>SGQDLVPAAVEQAVPIQPVAGAALAAPAAGQINQIDPWIFQNFVQCPLGEFSISPRNTPGEILFDLALGPGLNPYLAHLSAMYTGWVGNMEVQLVLAGNAFTAGKVVVALVPPYFPKGSLTTAQITCFPHVMCDVRTLEPIQLPLLDVRRVLWHATQDQEESMRLVCMLYTPLRTNSPGDESFVVSGRLLSKPAADFNFVYLTPPIERTIYRMVDLPVIQPRLCTHARWPAPVYGLLVDPSLPSNPQWQNGRVHVDGTLLGTTPISGSWVSCFAAEAAYEFQSGTGEVATFTLIEQDGSAYVPGDRAAPLGYPDFSGQLEIEVQTETTKTGDKLKVTTFEMILG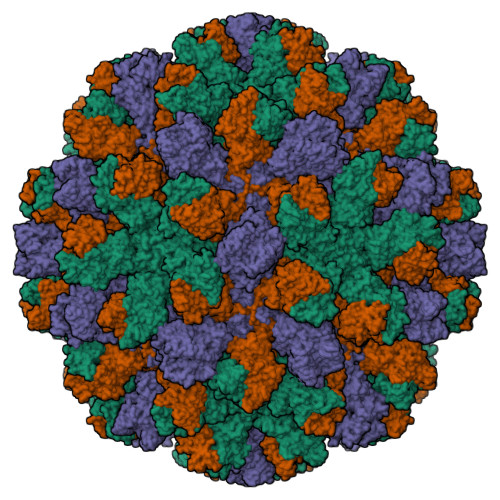PTTNADQAPYQGRVFASVTAAASLDLVDGRVRAVPRSIYGFQDTIPEYNDGLLVPLAPPIGPFLPGEVLLRFRTYMRQIDTADAAAEAIDCALPQEFVSWFASNAFTVQSEALLLRYRNTLTGQLLFECKLYNEGYIALSYSGSGPLTFPTDGIFEVVSWVPRLYQLASVGS[3x]>MVYVAVLANIAGNLPALTAALSRIEEMREEGYEIEKYYILGNIVGLFPYPKEVIEVIKDLTKKENVKIIRGKYDQIIAMSDPHATDPGYIDKLELPGHVKKALKFTWEKLGHEGREYLRDLPIYLVDKIGGNEVFGVYGSPINPFDGEVLAEQP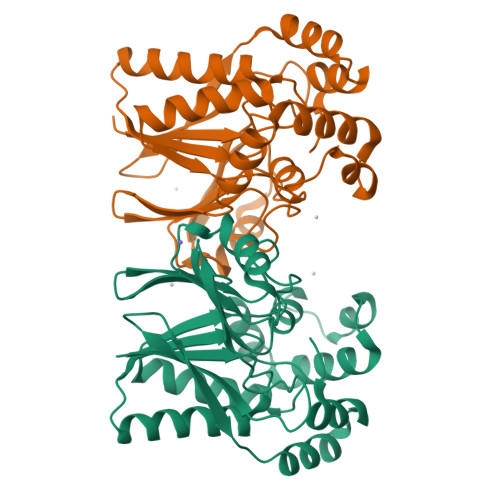TSYYEAIMRPVKDYEMLIVASPMYPVDAMTRYGRVVCPGSVGFPPGKEHKATFALVDVDTLKPKFIEVEYDKKIIEERIRAEGLPEEIIKILYHGGRP[2x]>[2x]MSTLIEAIVAREVLDSRGNPTIEVDVRLESGDVGRAIVPSGASTGAHEALELRDGDKSRYNGKGVLKAVQAVNEDIAEALIGFDAADQIALDQELIALDGTPNKSKLGANAILGVSLAAAKAAAAAFGLPLYRYLGGVYAHVLPVPMMNIMNGGQHATNSTDFQEFMIMPVGAESFREGLRWGAEIYHM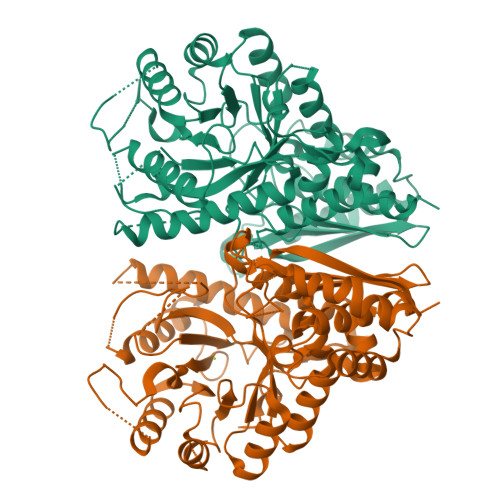LKKVIHDRGFSTTVGDEGGFAPSLPTNDAPLQLIMEAIEKAGYRPGEQIVIALDPATTEIFEDGKYHLKREGRSLSSAEMVDYWVDLVNRYPIISLEDGLAEDDWEGWALLRAKLGDRVQLVGDDFLVTNVQRLQRAIEAKAANSILIKLNQIGSLTETLSAIQLAQRSGWTAVVSHRSGESEDVTIADLVVATNAGQIKTGAPARTDRIAKYNQLLRIEEELGSAARYAGRSAFKV>MSHHHHHHSMDMTSKKRARDEEAQSGGSEAETKPAPVKKAKSKASNPGGSQVDAEGNPFWEISDKRRVGISQFKKMDFINIREYYEAGGEMKPGKKGIGLTVDQYTAFLKAIPAINAELRSRGHDITDDSDGGGAPVVAK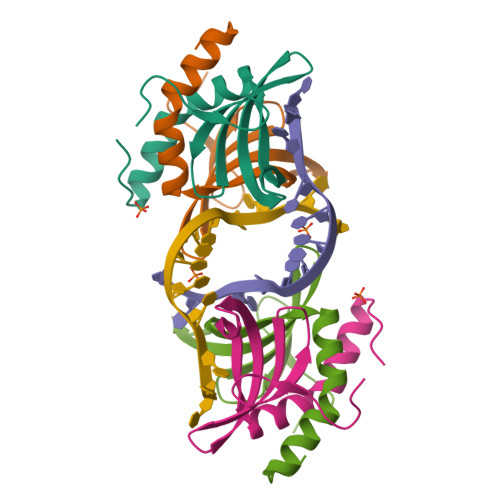PEGNAKKSTKKQEKKANIEATSDEGSGSD[2x]7-NITROINDAZOLE | C7 H5 N3 O2 | 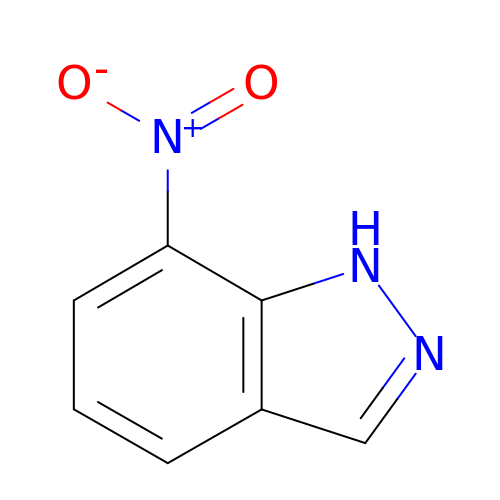PQCAUHUKTBHUSA-UHFFFAOYSA-N ethyl (2S)-2-[3-(benzenecarbonyl)phenyl]propanoate | C18 H18 O3 | 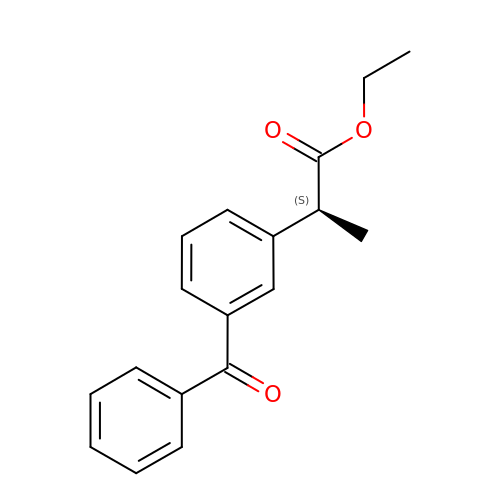CQSMNXCTDMLMLM-ZDUSSCGKSA-N> GPGHMVVKFSYMWTINNFSFCREEMGEVIKS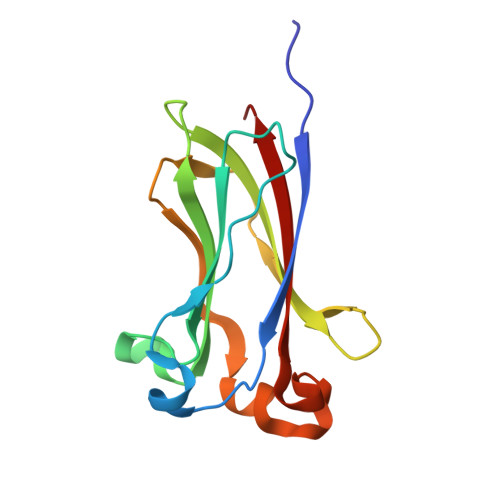STFSSGANDKLKWCLRVNPKGLDEESKDYLSLYLLLVSCPKSEVRAKFKFSILNAKGEETKAMEAQRAYRFVQGKDWGFKKFIRRDFLLDEANGLLPDDKLTLFCEVSVVQD> SINWPPEFHPGVPWKG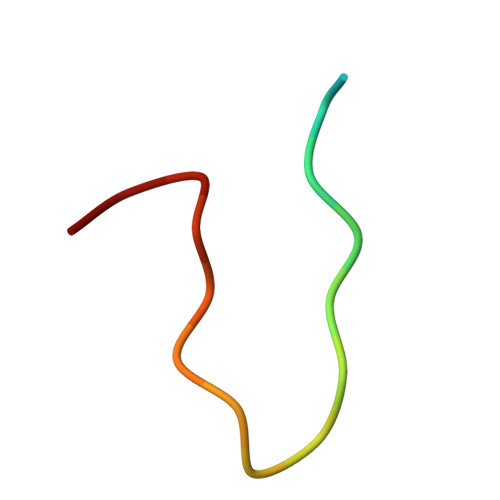LQ>[3x]MEEVKKDVYSVWALPDEESEPRFKKLMEALRSEFTGPRFVPHVTVAVSAYLTADEAKKMFESACDGLKAYTATVDRVSTGTFFF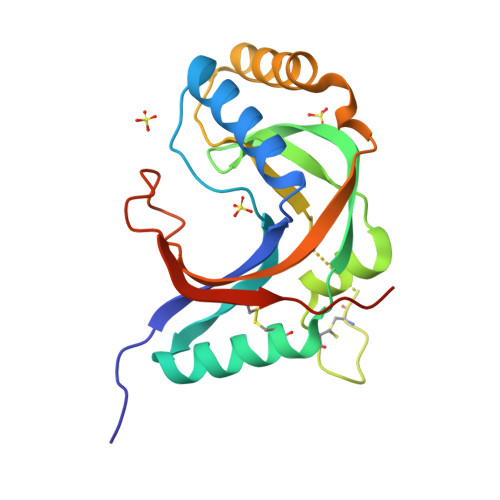QCVFLLLQTTPEVMEAGEHCKNHFNCSTTTPYMPHLSLLYAELTEEEKKNAQEKAYTLDSSLDGLSFRLNRLALCKTDTEDKTLETWETVAVCNLNPGSHHHHHH> MVNEGPNQEESDDTPVPESALQADPSVSVHPSVSVHPSVSINPSVSVHPSSSAHPSALAQPSGLAHPSSSGPEDL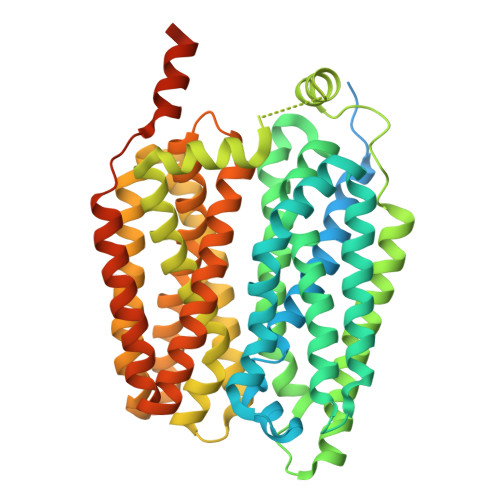SVIKVSRRRWAVVLVFSCYSMCNSFQWIQYGSINNIFMHFYGVSAFAIDWLSMCYMLTYIPLLLPVAWLLEKFGLRTIALTGSALNCLGAWVKLGSLKPHLFPVTVVGQLICSVAQVFILGMPSRIASVWFGANEVSTACSVAVFGNQLGIAIGFLVPPVLVPNIEDRDELAYHISIMFYIIGGVATLLLILVIIVFKEKPKYPPSRAQSLSYALTSPDASYLGSIARLFKNLNFVLLVITYGLNAGAFYALSTLLNRMVIWHYPGEEVNAGRIGLTIVIAGMLGAVISGIWLDRSKTYKETTLVVYIMTLVGMVVYTFTLNLGHLWVVFITAGTMGFFMTGYLPLGFEFAVELTYPESEGISSGLLNISAQVFGIIFTISQGQIIDNYGTKPGNIFLCVFLTLGAALTAFIKADLRRQKANKETLENKLQEEEEESNTSKVPTAVSEDHLDYKDDDDK>NPYLFESAGFASAFRTGEGHLKILEKFTQRSELFRGIEKYRVAVLEFEPQSFMVPNHCDGEVIY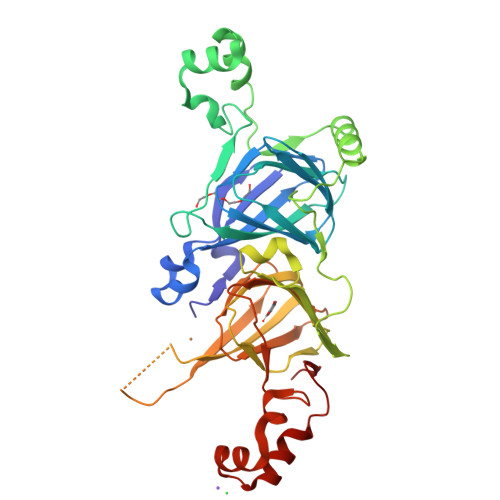VVAKGAGIISIAEQKAKYYFVLKKADVKRVPAGATIYFVNRDANQKLVVYVLVKSTNAPGEAQEYFSGGGQNPESFYRAFSSDILEKAFNTAADRLERLFGQQKQGPVIKASEEQIRAISQYASEPTAATGGEIRGPFNLLKGAPLFESRFGQFFEASPELFAQLRDLDVAVGYMNINQGGMVLPYYNTKSTRLVMVIEGNGRFEMACPHXXXXXXXXXXXXXXXXXXXXAGDVHYQKVRGNLNVGDLLVVPAAHPITFTATGGSNLRMVGFGINAQNNKKKFLAGKQNIWRNVDREAKELSFNMPGREVEEIFQKQDESYFVAGP[2x]>MKYNAPNTTPSSIGPQIRLDYYYKKALVDAAKEMYFGQLAEVTNMPKNMGKQIKLYHYVPLLDDRNVNDQGIDAAGATIANGNLYGSSKDIGTIPSKLPALTENGGRVNRVGFTRIQLIGSIKKFGFFYEWTQEAMDFDTDEELDSHLIQEAVKGANEITEDQLQIDLLNGAGVVRYPGAATSNADMTGEGTATVVTYEGLVKMGITLNDNLCPMQTKLIAGSLMTDTRTIQGARALYIGSELELQLRKMKDPFDNAAF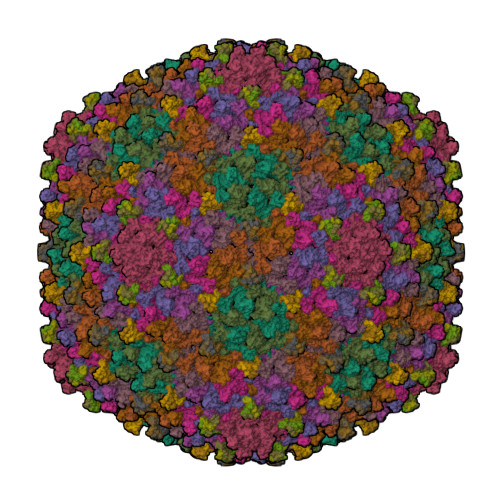IPVQQYADAGNLLKGEIGSIASFRVIVVPKMLKWAGAGATVTTNPGYYATSGKYDVFPMLCVGSGSFTTIGFQTDGKTVKFTTYTKKPGIETVSYADPYGEMGLTSIKWYYGSLILRPEWIALFKTVAAM[9x];>[9x]MAYSDVDAILADGKQAVAVKHGGGLVVVGELGAQVLAAKDVSELPDGVGGTAPGAATTTTAGVVKQSTTQAASVATDVAGVVTDLNALITKLKAAGIMA> MMKGSRRTGNNTATTLNTPVVIHATQLPQHVSTDEVLQFL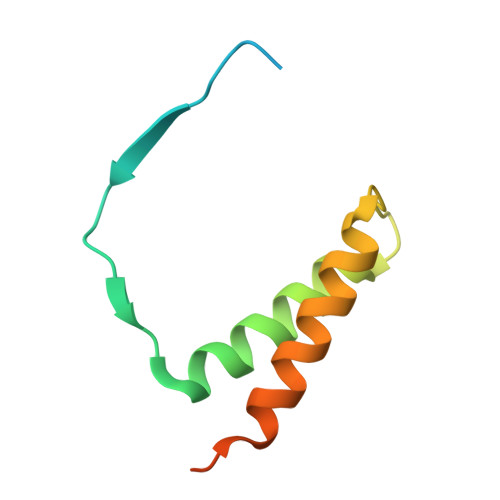ESFIDEKENIIDIDTNLSSSISQLKRIQRDFKGLPPAQDFSAAPIQV>FQYIITEKKGKNSSVGLIQLNRPKALNA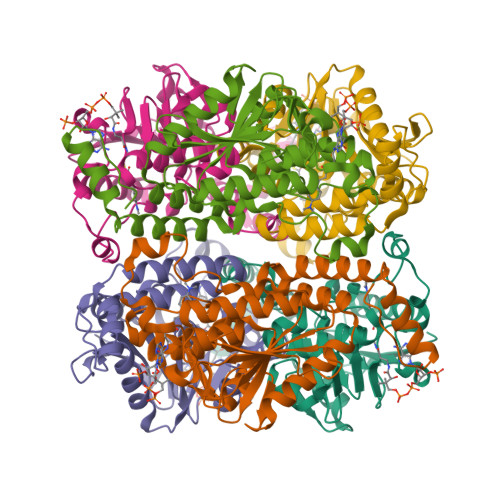LCNGLIEELNQALETFEEDPAVGAIVLTGGEKAFAAGADIKEMQNRTFQDCYSGKFLSHWDHITRIKKPVIAAVNGYALGGGCELAMMCDIIYAGEKAQFGQPEILLGTIPGAGGTQRLTRAVGKSLAMEMVLTGDRISAQDAKQAGLVSKIFPVETLVEEAIQCAEKIANNSKIIVAMAKESVNAAFEMTLTEGNKLEKKLFYSTFATDDRREGMSAFVEKRKANFKDH[6x]> MTTTKTFDERNRDTQDGFERHVFRKLDHTDTGAIVTVEGSGTMDEDVPVINSGYGFNPEDDEELEVFLLSDGSDASGKFGVMTIPRNKQRKWPKKTGGIQHPFNADKFVQLDDDSIWLKDGKFTLGDNRSLSITVEGNNVVIDTGGGELDIRSSKLMHNGVNIGDSHVHPQQAD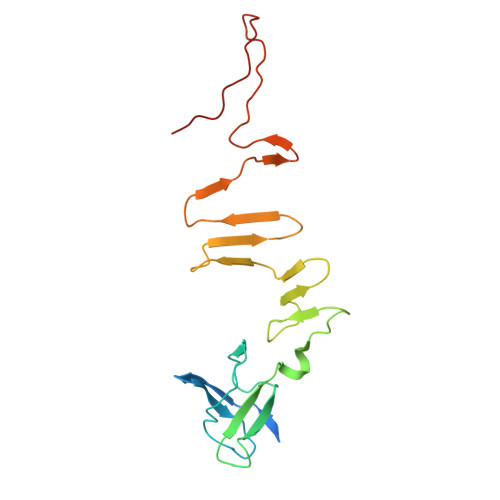SDGDTEADTDPPKRD pyrene | C16 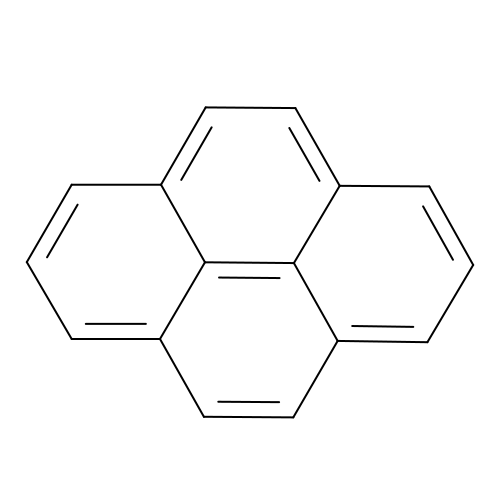H10 | BBEAQIROQSPTKN-UHFFFAOYSA-N> GSHMASLTEIEHLVQSV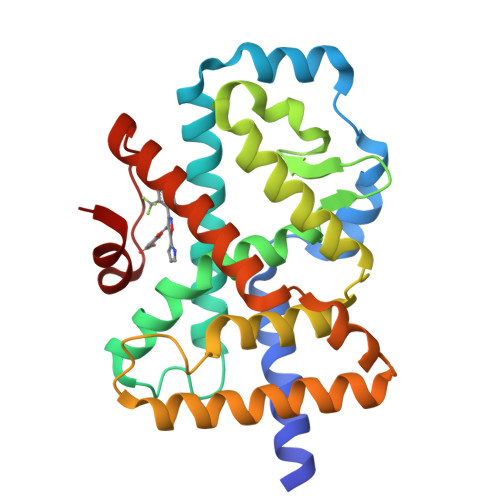CKSYRETCQLRLEDLLRQRSNIFSREEVTGYQRKSMWEMWERCAHHLTEAIQYVVEFAKRLSGFMELCQNDQIVLLKAGAMEVVLVRMCRAYNADNRTVFFEGKYGGMELFRALGCSELISSIFDFSHSLSALHFSEDEIALYTALVLINAHRPGLQEKRKVEQLQYNLELAFHHHLHKTHRQSILAKLPPKGKLRSLCSQHVERLQIFQHLHPIVVQAAFPPLYKELFS>[4x]ACDYTCGSNCYSSSDVSTAQAA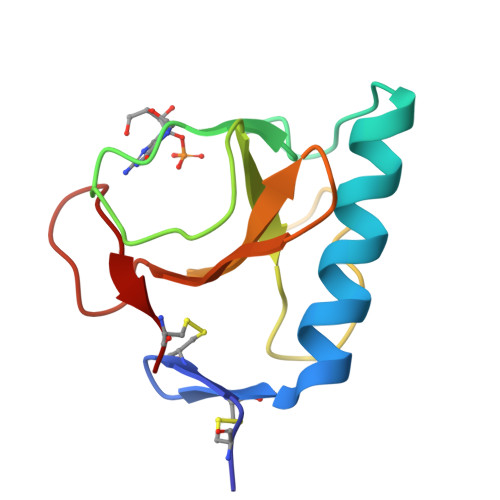GYKLHEDGETVGSNSYPHKYNNYEGFDFSVSSPYYEWPILSSGDVYSGGSPGADRVVFNENNQLAGVITHTGASGNNFVECT> MDIVISGTRVIYKSDQKSVNVRLENKGNNPLLVQSWLDTGDDNAEPGSITVPFTATPPVSRIDAKRGQTIKLMYTASTSLPKDRESVFWFNVLEVPPKPDAEKVANQSLLQLAFRTRIKLFYRPDGLKGNPSEAPLALKWFWSGSEGKASLRVTN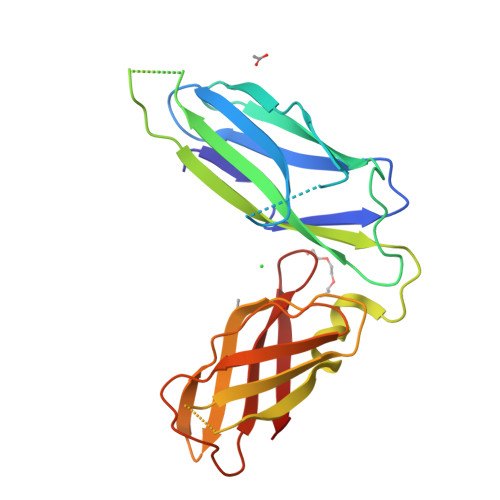PTPYYVSFSSGDLEASGKRYPIDVKMIAPFSDEVMKVNGLNGKANSAKVHFYAINDFGGAIEGNARL>MDTIVKKTRTRLSPEKRKQQLLDYALDVFARRGIGRAGHADIAEMANVSVATVFNYFPTREALVEQVLTQVENRFSTMLQTCMGNPGKPLLLRLNCITHNLIDAVIEQQDWLKVWFEWSTSIRDEIWPQFTHDNRKSLECLTEMFAEGLEKQEITTQQPADKLAWQLYGICYVLYLQANLNPDQEQM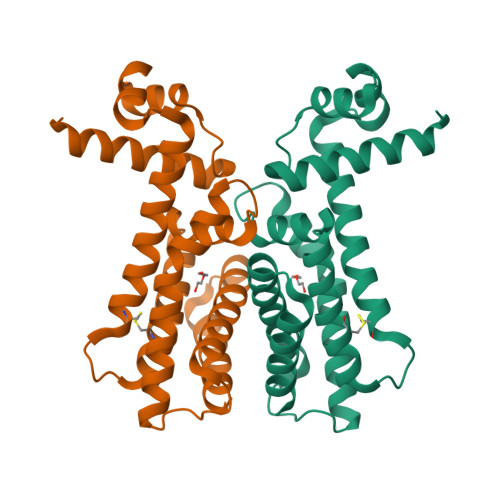RELADGYVTGLLGK[2x]>[2x]GTLDTTWKEATLPQVKAMLQKDTGKVSGDTVTYSGKTVHVVAAAVLPGFPFPSFEVHDKKNPTLQIPAGATVDVTFINTNKGFGHDFDITKKGPP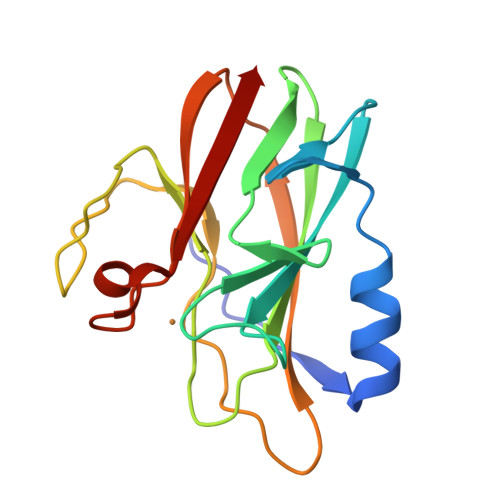YAVMPVIDPIVAGTGFSPVPKDGKFGYTNFTWHPTAGTYYYVCQIPGHAATGMFGKIVVK> SASIWVGHRGTVRDYPDFSPSVDAEAIQKAIRGIGTDEKMLISILTERSNAQRQLIVKEYQAAYGKELKDDLKGDLSGHFEHLMVALVTPPAVFDAKQLKKSMKGAGTNEDALIEILTTRTSRQMKDISQAYYTVYKKSLGDDISSETSGDFRKALLTLADGRRDESLKVDEHLAKQDAQILYKAGENRWGTDEDKFTEILCLRSFPQLKLTFDEYRNISQKDIVDSIKGELSGHFEDLLLAIVNCVRNTPAFLAERLHRALKGIGTDEFTLNRIMVSRSEIDLLDIRTEFKKHY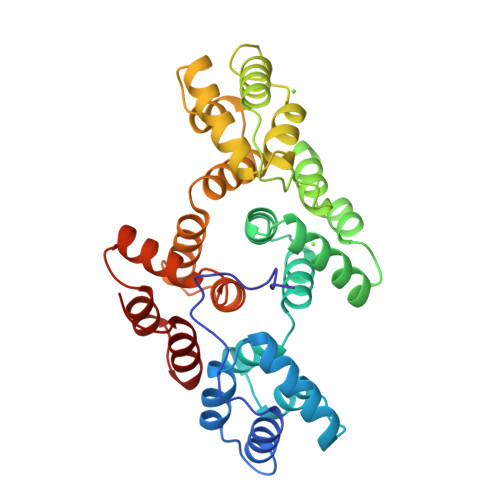GYSLYSAIKSDTSGDYEITLLKICGGDD> GIPMETKGGTVKAASGFNATEDAQVLRKAMKGLGTDEDAIIGVLACRNTAQRQEIRTAYKSTIGRDLLEDLKSELSSNFEQVILGMMTPTVLYDVQELRRAMKGAGTDEGCLIEILASRNPEEIRRINQTYQQQYGRSLEEDICSDTSFMFQRVLVSLTAGGRDEGNYLDDALVKQDAQDLYEAGEKRWGTDEVKFLSILCSRNRNHLLHVFDEYKRISQKDIEQSIKSETSGSFEDALLAIVKCMRNKPAYFAERLYKSMKGLGTDDSTLIRVMVSRAEI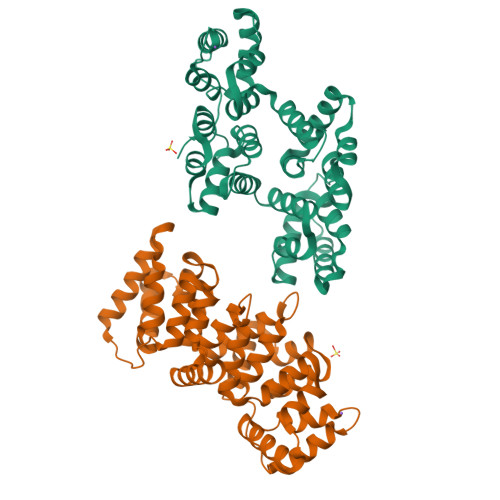DMLDIRANFKRLYGKSLYSFIKGDTSGDYRKVLLILCGGDD>MAAPVVAPPGVVVSRANKRSGAGPGGSGGGGARGAEEEPPPPLQAVLVADSFDRRFFPISKDQPRVLLPLANVALIDYTLEFLTATGVQETFVFCCWKAAQIKEHLLKSKWCRPTSLNVVRIITSELYRSLGDVLRDVDAKALVRSDFLLVYGDVISNINITRALEEHRLRRKLEKNVSVMTMIFKESSPSHPTRCHEDNVVVAVDSTTNRVLHFQKTQGLRRFAFPLSLFQGSSDGVEVRYDLLDCHISICSPQVAQLFTDNFDYQTRDDFVRGLLVNEEILGNQIHMHVTAKEYGARVSNLHMYSAVCADVIRRWVYPLTPEANFTDSTTQSCTHSRHNIYRGPEVSLGHGSILEENVLLGSGTVIGSNCFITNSVIGPGCHIGDNVVLDQTYLWQGVRVAAGAQIHQSLLCDNAEVKERVTLKPRSVLTSQVVVGPNITLPEGSVISLHPPDAEEDEDDGEFSDDSGADQEKDKVKMKGYNPAEVGAAGKGYLWKAAGMNMEEEEELQQNLWGLKINMEEESESESEQSMDSEEPDSRGGSPQMDDIKVFQNEVLGTLQRGKEENISCDNLVLEINSLKYAYNVSLKEVMQVLSHVVLEFPLQQMDSPLDSSRYCALLLPLLKAWSPVFRNYIKRAADHLEALAAIEDFFLEHEALGISMAKVLMAFYQLEILAEETILSWFSQRDTTDKGQQLRKNQQLQRFIQWLKEAEEESSEDD[2x];>MHHHHHHGGGSENLYFQSPGSAAKGSELSERIESFVETLKRGGGPRSSEEMARETLGLLRQIITDHRWSNAGELMELIRREGRRMTAAQPSETTVGNMVRRVLKIIREEYGRLHGRSDESDQQESLHKLLTSGGLNEDFSFHYAQLQSNIIEAINELLVELEGTMENIAAQALEHIHSNEVIMTIGFSRTVEAFLKEAARKRKFHVIVAECAPFCQGHEMAVNLSKAGIETTVMTDAAIFAVMSRVNKVIIGTKTILANGALRAVTGTHTLALAAKHHSTPLIVCAPMFKLSPQFPNEEDSFHKFVAPEEVLPFTEGDILEKVSVHCPVFDYVPPELITLFISNIGGNAPSYIYRLMSELYHPDDHVL[2x];>MAAVAVAVREDSGSGMKAELPPGPGAVGREMTKEEKLQLRKEKKQQKKKRKEEKGAEPETGSAVSAAQCQVGPTRELPESGIQLGTPREKVPAGRSKAELRAERRAKQEAERALKQARKGEQGGPPPKASPSTAGETPSGVKRLPEYPQVDDLLLRRLVKKPERQQVPTRKDYGSKVSLFSHLPQYSRQNSLTQFMSIPSSVIHPAMVRLGLQYSQGLVSGSNARCIALLRALQQVIQDYTTPPNEELSRDLVNKLKPYMSFLTQCRPLSASMHNAIKFLNKEITSVGSSKR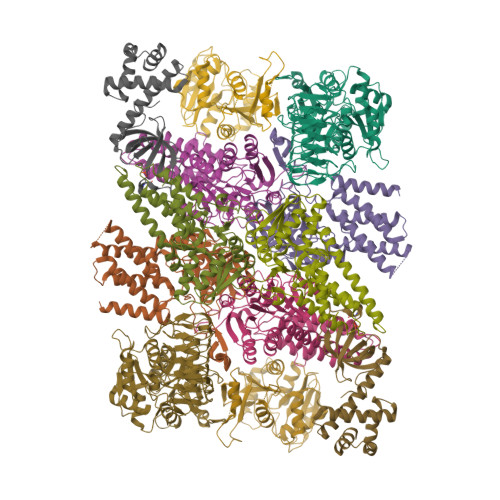EEEAKSELRAAIDRYVQEKIVLAAQAISRFAYQKISNGDVILVYGCSSLVSRILQEAWTEGRRFRVVVVDSRPWLEGRHTLRSLVHAGVPASYLLIPAASYVLPEVSKVLLGAHALLANGSVMSRVGTAQLALVARAHNVPVLVCCETYKFCERVQTDAFVSNELDDPDDLQCKRGEHVALANWQNHASLRLLNLVYDVTPPELVDLVITELGMIPCSSVPVVLRVKSSDQ[2x];>[2x]MDDKELIEYFKSQMKEDPDMASAVAAIRTLLEFLKRDKGETIQGLRANLTSAIETLCGVDSSVAVSSGGELFLRFISLASLEYSDYSKCKKIMIERGELFLRRISLSRNKIADLCHTFIKDGATILTHAYSRVVLRVLEAAVAAKKRFSVYVTESQPDLSGKKMAKALCHLNVPVTVVLDAAVGYIMEKADLVIVGAEGVVENGGIINKIGTNQMAVCAKAQNKPFYVVAESFKFVRLFPLNQQDVPDKFKYKADTLKVAQTGQDLKEEHPWVDYTAPSLITLLFTDLGVLTPSAVSDELIKLYL;>MEFQAVVMAVGGGSRMTDLTSSIPKPLLPVGNKPLIWYPLNLLERVGFEEVIVVTTRDVQKALCAEFKMKMKPDIVCIPDDADMGTADSLRYIYPKLKTDVLVLSCDLITDVALHEVVDLFRAYDASLAMLMRKGQDSIEPVPGQKGKKKAVEQRDFIGVDSTGKRLLFMANEADLDEELVIKGSILQKHPRIRFHTGLVDAHLYCLKKYIVDFLMENGSITSIRSELIPYLVRKQFSSASSQQGQEEKEEDLKKKELKSLDIYSFIKEANTLNLAPYDACWNACRGDRWEDLSRSQVRCYVHIMKEGLCSRVSTLGLYMEANRQVPKLLSALCPEEPPVHSSAQIVSKHLVGVDSLIGPETQIGEKSSIKRSVIGSSCLIKDRVTITNCLLMNSVTVEEGSNIQGSVICNNAVIEKGADIKDCLIGSGQRIEAKAKRVNEVIVGNDQLMEI[2x];>[2x]MDYKDDDDKPGLSCRFYQHKFPEVEDVVMVNVRSIAEMGAYVSLLEYNNIEGMILLSELSRRRIRSINKLIRIGRNECVVVIRVDKEKGYIDLSKRRVSPEEAIKCEDKFTKSKTVYSILRHVAEVLEYTKDEQLESLFQRTAWVFDDKYKRPGYGAYDAFKHAVSDPSILDSLDLNEDEREVLINNINRRLTPQAVKIRADIEVACYGYEGIDAVKEALRAGLNCSTENMPIKINLIAPPRYVMTTTTLERTEGLSVLSQAMAVIKEKIEEKRGVFNVQMEPKVVTDTDETELARQMERLERENAEVDGDDDAEEMEAKAED> GGLRRRDLPADPLTLFERWLSQACEAKLADPTAMVVATVDEHGQPYQRIVLLKHYDEKGMVFYTNLGSRKAHQIENNPRVSLLFPWHTLERQVMVIGKAERLSTLEVMKYFHSRPRDSQIGAWVSKQSSRISARGILESKFLELKQKFQQGEVPLPSFWGGFRVSLEQIEFWQGGEHRLHDRFLYQRE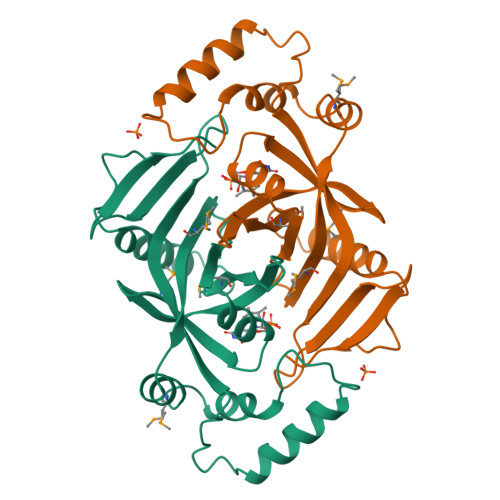NDAWKIDRLAP>MSLRIGVIGTGAIGKEHINRITNKLSGAEIVAVTDVNQEAAQKVVEQYQLNATVYPNDDSLLADENVDAVLVTSWGPAHESSVLKAIKAQKYVFCEKPLATTAEGCMRIVEEEIKVGKRLVQVGFMRRYDSGYVQLKEALDNHVIGEPLMIHCAHRNPTVGDNYTTDMAVVDTLVHEIDVLHWLVNDDYESVQVIYPKKSKNALPHLKDPQIVVIETKGGIVINAEIYVNCKYGYDIQCEIVGEDGIIKLPEPSSISLRKEGRFSTDILMDWQRRFVAAYDVEIQDFIDSIQKKGEVSGPTAWD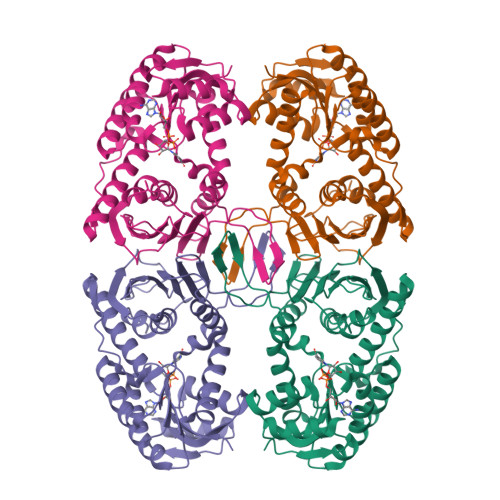GYIAAVTTDACVKAQESGQKEKVELKEKPEFYQSFTTVQN[2x]>MAADLRAPLTPAGRTVVDLLAGVIPRISAEAADRDRTGTFPVEAFEQFAKLGLMGATVPAELGGLGLTRLYDVATALMRLAEADASTALAWHVQLSRGLTLTYEWQHGTPPVRAMAERLLRAMAEGEAAVCGALKDAPGVVTELHSDGAGGWLLSGRKVLVSMAPIATHFFVHAQRRDDDGSVFLAVPVVHRDAPGLTVLDNWDGLGMRASGTLEVVFDRCPVRADELLERGPVGARRDAVLAGQTVSSITMLGIYAGIAQAARDIAVGFCAGRGGEPRAGARALVAGLDTRLYALRTTVGAALTNADAASVDLSGD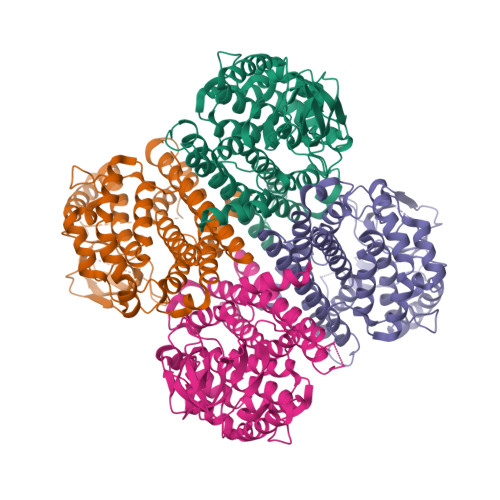PDERGRRMMTPFQYAKMTVNELAPAVVDDCLSLVGGLAYTAGHPLSRLYRDVRAGGFMQPYSYVDAVDYLSGQALGLD[4x]>MSNYYYYYGGGRYDWLKTVEPTNFLKIGLPYQAHPLHLQHQATTPPSILEKFKRADILLNEVKAEMDPLMLQPETEKKLFQILSSIDMFKGLRKKVEFTYNAQIVTNAWLKMYELLNTMNFNNTSQAFCNCELPGGFISAINHFNYTMMHYPTFNWVASSLYPSSETDALEDHYGLYQCNPDNWLMQSPLLKKNIDYNNGDVTIASNVKNLALRATQRLTPIHLYTADGGINVGHDYNKQEELNLKLHFGQALTGLLSLSKGGNMILKHYTLNHAFTLSLICVFSHFFEELYITKPTSSRPTNSETYIVGKNRLRLFTPKEEQVLLKRLEFFNDTPLVDLSLYQNLLESVYFAV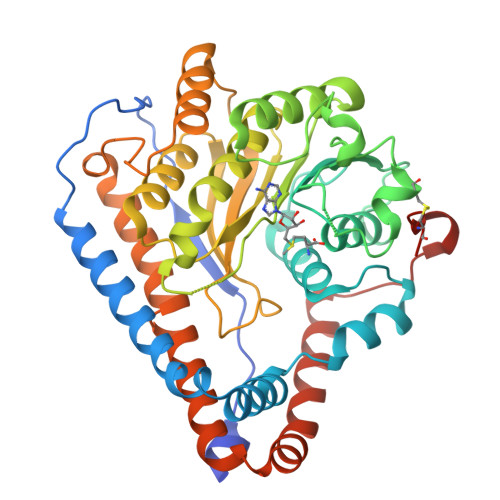ETIHLKQQIEFLNFGMKCYRHFYNKIKLLNDYLAPKKKIFQDRWRVLNKLYVLEKKHKLKLCASHHHHHHHH[2x]1-methyl-5-oxidanyl-4-oxidanylidene-pyridine-2-carboxylic acid | C7 H7 N O4 | 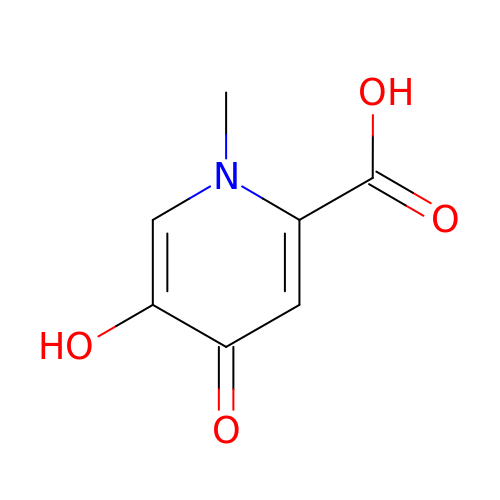XWHROGRDGWNCHV-UHFFFAOYSA-N>[4x]RLTELREDIDAILEDPALEGAVSGVVVVDTATGEELYSRDGGEQLLPASNMKLFTAAAALEVLGADHSFGTEVAAESAPGRRGEVQDLYLVGRGDPTLSAEDLDAMAAEVAASGVRTVRGDLYADDTWFDSERLVDDWWPEDEPYAYSAQISALTV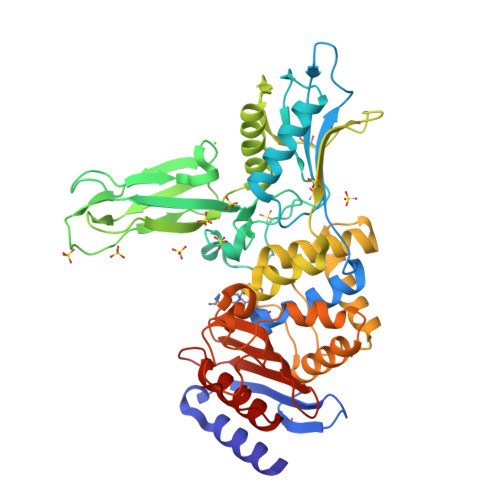AHGERFDTGVTEVSVTPAAEGEPADVDLGAAEGYAELDNRAVTGAAGSANTLVIDRPVGTNTIAVTGSLPADAAPVTALRTVDEPAALAGHLFEEALESNGVTVKGDVGLGGVPADWQDAEVLADHTSAELSEILVPFMKFSNNGHAEMLVKSIGQETAGAGTWDAGLVGVEEALSGLGVDTAGLVLNDGSGLSRGNLVTADTVVDLLGQAGSAPWAQTWSASLPVAGESDPFVGGTLANRMRGTAAEGVVEAKTGTMSGVSALSGYVPGPEGELAFSIVNNGHSGPAPLAVQDAIAVRLAEYAGHQAPE> MASMTGGQQMGRDQAGITGTWYNQLGSTFIVTAGAD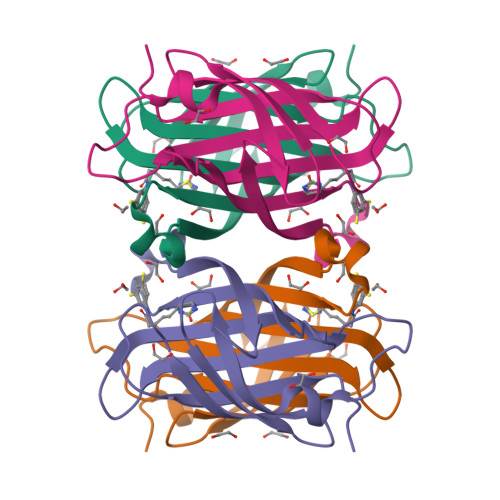GALTGTYESAVGNAESRYVLTGRYDSAPATDGSGTALGWTVAWKNNYRNAHSATTWSGQYVGGAEARINTQWLLTSGTTEANAWKSTLVGHDTFTKVKPSAASIDAAKKAGVNNGNPLDAVQQ> DLQLLHQKVEEQAAKY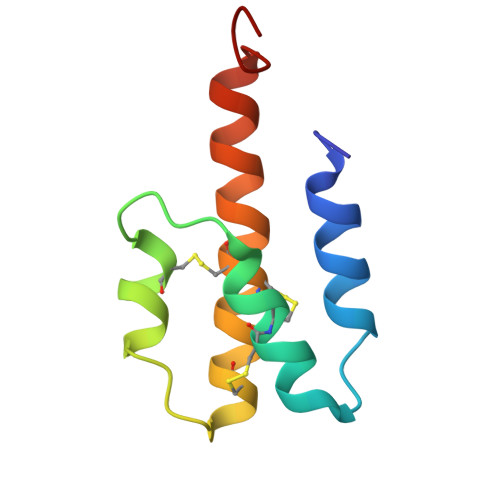KHRVPKKCCYDGARENKYETCEQRVARVTIGPHCIRAFNECCTIADKIRKESHHKGMLLGR>IQLIPPLINLLMSIEPDVIYAGHDNTKPDTSSSLLTSLNQLGERQLLSVVKWSKSLPGFRNLHIDDQITLIQYSWMSLMVFGLGWRSYKHVSGQMLYFAPDLILNEQRMKESSFYSLCLTMWQIPQEFVKLQVSQEEFLCMKVLLLLNTIPLEGLRSQTQFEEMRSSYIRELIKAIGLRQKGVVSSSQRFYQLTKLLDNLHDLVKQLHLYCLNTFIQSRALSVEFPEMMSEVIAAQLPK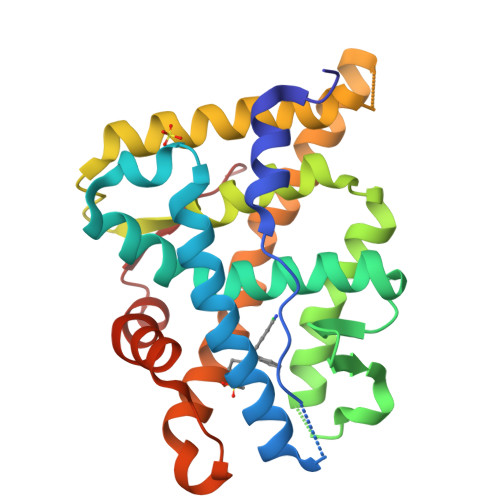ILAGMVKPLLFHKK[2x]> MTQPLTGTTPAAGGYTTV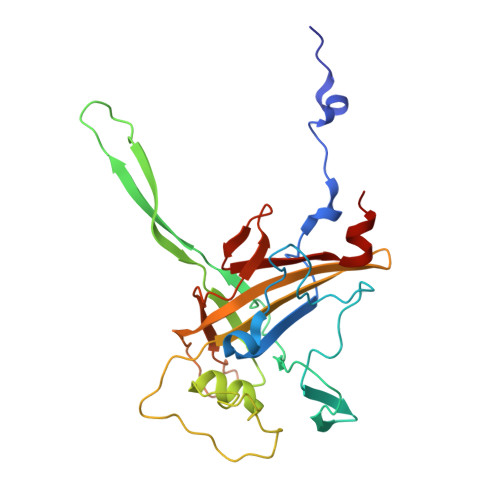DNRLQGGHRTGLIAVAFRDALGTSTNISPHNANGSVRWSPLAQDGQLRDDLFAHRLENGVWVENTNPNEGWYLAGAFGEGNGPSSRPSIDTDDQMIEQSNWPFESDITKQDEPFTFQALQNLYPAIQRLANNLPLSDANGNPLVELPGEADGFSQPVDAEKIGRQFLLYGIRKKEGRYLYEVDAYDLAYLNNKGERKFGKRGTAAELTFKPEPSGYFMAMVDGEYKPIIKHTFIGGPAWDALAGDGS> AFGITTSSSAYVIDTNAPNQLKFTVSRSSCDITSIIHYGTELQYSSQGSHIGSGLGSATVTATQSGDYIKVTCVTDTLTQYMVVHNGDPIIHMATYITAEPSIGELRFIARLNSDLLPNEEPFGDVSTTADGTAIEGSDVF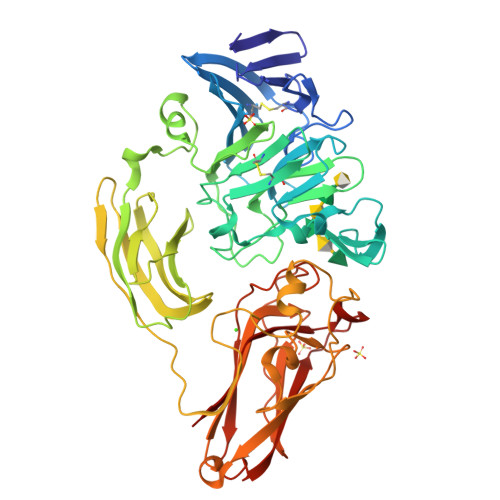LVGSETRSAFYSSERFIDDQRHCIAGDAHRVCMILNQYESSSGGPFHRDINSNNGGSYNALYWYMNSGHVQTESYRMGLHGPYSMYFSRSGTPSTSIDTSFFADLDIKGYVAASGRGKVAGTASGADSSMDWVVHWYNDAAQYWTYTSSSGSFTSPAMKPGTYTMVYYQGEYAVATSSVTVSAGSTTTKNISGSVKTGTTIFKIGEWDGQPTGFRNAANQLRMHPSDSRMSSWGPLTYTVGSSALTDFPMAVFKSVNNPVTIKFTATSAQTGAATLRIGTTLSFAGGRPQATINSYTGSAPAAPTNLDSRGVTRGAYRGLGEVYDVSIPSGTIVAGTNTITINVISGSSGDTYLSPNFIFDCVELFQ>[3x]IVHREHQESQEESDSRGENNPFYFSSDRRFHTLFTNQYGHLRILHRFDQRSKQIQNLENYRVVEFKSKPNTLLLPHHADADFLLVVLNGRAILT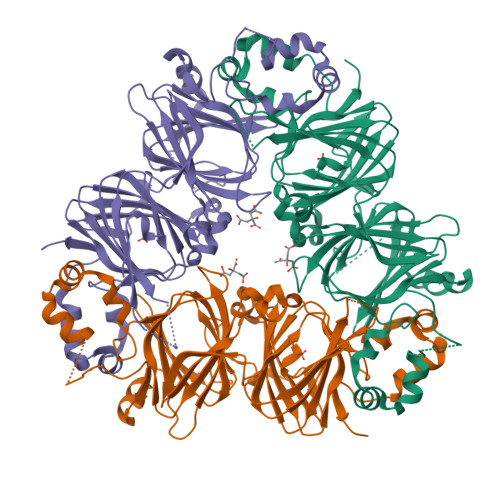LVNPDSRDSYILEQGHAQKIPAGTTFFLVNPDDNENLRIIKLAIPVNNPHRFQDFFLSSTEAQQSYLRGFSKNILEASFDSDFKEINRVLFGEERQQQQGEESREEGVIVELKREQIQELMKHAKSSSRKELSSQDEPFNLRNSKPIYSNKFGRWYEMTPEKNPQLKDLDVFISSVDMKEGALLLPHYNSKAIVIMVINEGEAKIELVGLSDQQQQKQQEESLEVQRYRAELSEDDVFVIPAAYPVAINATSNLNFFAFGINAENNQRNFLAGGKDNVMSEIPTEVLEVSFPASGKKVEKLIKKQSESHFVDAQPEQQQREEGHKGRKGSLSSILGSLY>[18x]MNPHDLEWLNRIGERKDIMLAVLLLAVVFMMVLPLPPIVLDILIAVNMTISVVLLMIAIYINSPLQFSAFPAVLLVTTLFRLALSVSTTRMILLQADAGQIVYTFGNFVVGGNLIVGIVIFLIITIVQFLVITKGSER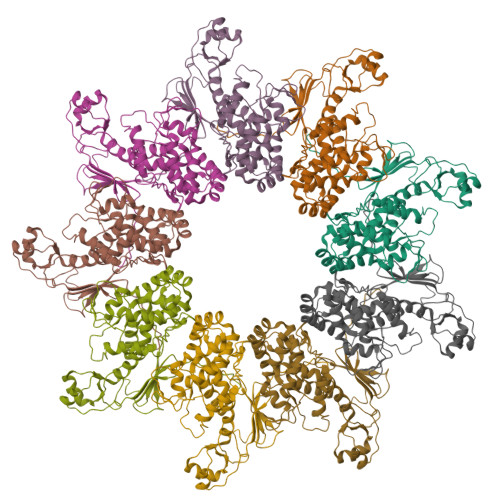VAEVSARFSLDAMPGKQMSIDGDMRAGVIDVNEARERRATIEKESQMFGSMDGAMKFVKGDAIAGLIIIFVNILGGVTIGVTQKGLAAAEALQLYSILTVGDGMVSQVPALLIAITAGIIVTRVSSEDSSDLGSDIGKQVVAQPKAMLIGGVLLLLFGLIPGFPTVTFLILALLVGCGGYMLSRKQSRNDEANQDLQSILTSGSGAPAARTKAKTSGANKGRLGEQEAFAMTVPLLIDVDSSQQEALEAIALNDELVRVRRALYLDLGVPFPGIHLRFNEGMGEGEYLISLQEVPVARGELKAGYLLVRESVSQLELLGIPYEKGEHLLPDQETFWVSVEYEERLEKSQLEFFSHSQVLTWHLSHVLREYAEDFIGIQETRYLLEQMEGGYGELIKEVQRIVPLQRMTEILQRLVGEDISIRNMRSILEAMVEWGQKEKDVVQLTEYIRSSLKRYICYKYANGNNILPAYLFDQEVEEKIRSGVRQTSAGSYLALDPAVTESLLEQVRKTIGDLSQIQSKPVLIVSMDIRRYVRKLIESEYYGLPVLSYQELTQQINIQPLGRVCLENLYFQ>MSTEPVSASDKYQKISQLEHILKRPDTYIGSVETQEQLQWIYDEETDCMIEKNVTIVPGLFKIFDEILVNAADNKVRDPSMKRIDVNIHAEEHTIEVKNDGKGIPIEIHNKENIYIPEMIFGHLLTSSNYDDDEKKVTGGRNGYGAKLCNIFSTEFILETADLNVGQKYVQKWENNMSICHPPKITSYKKGPSYTKVTFKPDLTRFGMKELDNDILGVMRRRVYDINGSVRDINVYLNGKSLKIRNFKNYVELYLKSLEKKRQLDNGEDGAAKSDIPTILYERINNRWEVAFAVSDISFQQISFVNSIATTMGGTHVNYITDQIVKKISEILKKKKKKSVKSFQIKNNMFIFINCLIENPAFTSQTKEQLTTRVKDFGSRCEIPLEYINKIMKTDLATRMFEIADANEENALKKSDGTRKSRITNYPKLEDANKAGTKEGYKCTLVLTEGDSALSLAVAGLAVVGRDYYGCYPLRGKMLNVREASADQILKNAEIQAIKKIMGLQHRKKYEDTKSLRYGHLMIMTDQDHDGSHIKGLIINFLESSFPGLLDIQGFLLEFITPIIKVSITKPTKNTIAFYNMPDYEKWREEESHKFTWKQKYYKGLGTSLAQEVREYFSNLDRHLKIFHSLQGNDKDYIDLAFSKKKADDRKEWLRQYEPGTVLDPTLKEIPISDFINKELILFSLADNIRSIPNVLDGFKPGQRKVLYGCFKKNLKSELKVAQLAPYVSECTAYHHGEQSLAQTII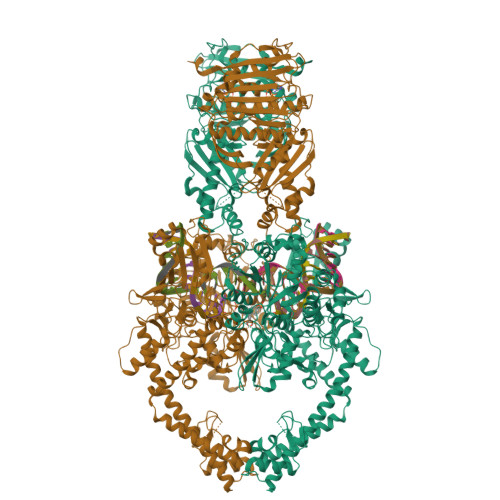GLAQNFVGSNNIYLLLPNGAFGTRATGGKDAAAARYIYTELNKLTRKIFHPADDPLYKYIQEDEKTVEPEWYLPILPMILVNGAEGIGTGWSTYIPPFNPLEIIKNIRHLMNDEELEQMHPWFRGWTGTIEEIEPLRYRMYGRIEQIGDNVLEITELPARTWTSTIKEYLLLGLSGNDKIKPWIKDMEEQHDDNIKFIITLSPEEMAKTRKIGFYERFKLISPISLMNMVAFDPHGKIKKYNSVNEILSEFYYVRLEYYQKRKDHMSERLQWEVEKYSFQVKFIKMIIEKELTVTNKPRNAIIQELENLGFPRFNKEGKPYYGSPNDEIAEQINDVKGATSDEEDEESSHEDTENVINGPEELYGTYEYLLGMRIWSLTKERYQKLLKQKQEKETELENLLKLSAKDIWNTDLKAFEVGYQEFLQRDAEAR[2x]> SRWQALFDD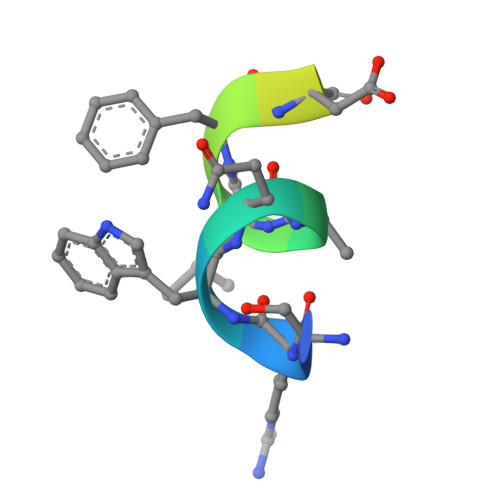GTDTSR>[2x]LVPRGSHMSIFDKRVNYKPFEYPEVLQFTEAINKAYWVHTEVDFTADTQDFHAHLSLAEKTAVKNSL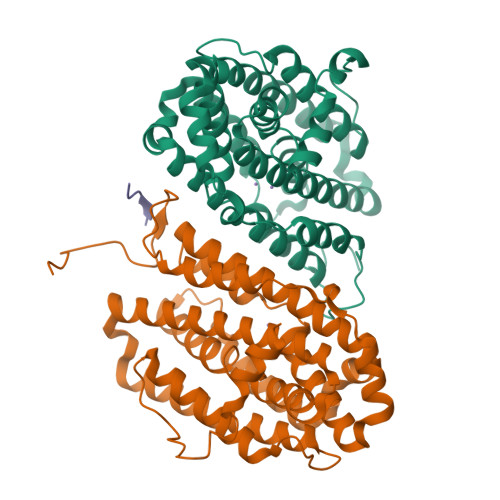LAIAQIEVAVKSFWGNIYEHFPKPEFNGLGSTFAECEFRHSEAYSRLLEVLGYNDEFEKLLDVPVIRRRVDYLSNVLKDTKSQDNRKYMVSLILFSILIENVSLFSQFAILLSFTRFKGYMKNVSNIIAWTSIDEQIHANGGIYIINKIREEFPDYFDEETLALVRETVKDSIAVESDILDWIFEEGEIESIKKGDLVNFMKFRIDESLKQINIPVIFDVKVEDYKALAWFEEEVFANSL;> VEYTKH> SVASRIHFLNSRTRFQTAVHASDVAPPFLLLPLASPRPLLAYHHRFRTRNRKRGSRFHPHPLPLPPPPLSPPRSDAAHLFAGKPLAASAVSTAAGQQTLPPPLLRHLQGLFPVFRGPECDPSCGVGPAGEAAGLALLPPPSLVEPRHLEDLARRALQARGETRDAASGACKSDRLFWRELAARVEKVRDLLPIESLVRLLTILTLNGASGTVRPVKQIFQAFETQDEDTPATPANRTGLRLASETLPCVRPLPPRLLLASTREFLEDLKKLSPPATAALAATFAWSNCASSALLFALMERWAWRQPRAEPSVQTDVESEVEPLGKRREAETGVEEEAENAKKLEAVETQGHLGDFTPADFA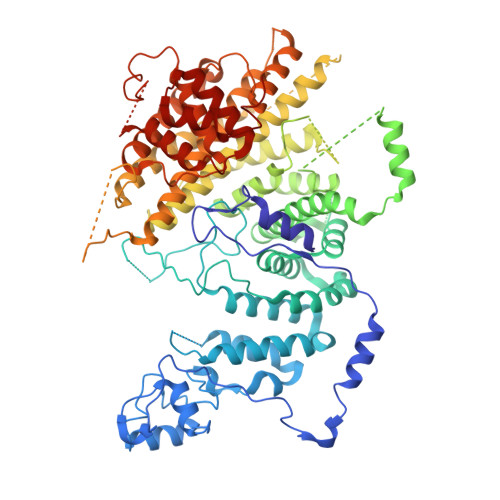LFVSALGHLLSQQEATHVKYSRQARHLREISGKQIMAAFREQKRQKGKQTADANFENFEETKSAWHFTAAFFDGCCRFMATRAESFSLFSFASAARTLVENLDAVALVGEAAESRALAVDGEGAGSVESLGIHGISTFSSFEGSVSRSEKPHVACPTPDSVEALAKAISLFVASWDGGDKTHGRLATRAANLLLVARLLRAASQCELYIHLHRALRLEAEGSGEGKSPQKRNSGEQASGAGVDDGGRGIAVDTVGACKTLLEHISCELGLLHSELEALPLLNSTLEDADDSADEKKAVDAPTERGFVHISPDTVYVRNELLAAAGESAAAVVRLHHAKSLLQATDEVARDSQSLRKGEAENVCHLSTGARVDRVKRWMRGQQAERMQLETLGELKSEAEHLADAIDRVLRERGAAGLPTEQLADLMEVFALCVGDKRVSQTPEETSRWFRLGLGDKAEKMNQANLSSLQALSSEIVRRYAALDVNQKRRIKWATRQMDWKDPYLNHCLGRFTAAVTRQR3-chloro-5-({1-[(4-methyl-5-oxo-4,5-dihydro-1H-1,2,4-triazol-3-yl)methyl]-2-oxo-4-(trifluoromethyl)-1,2-dihydropyridin-3-yl}oxy)benzonitrile 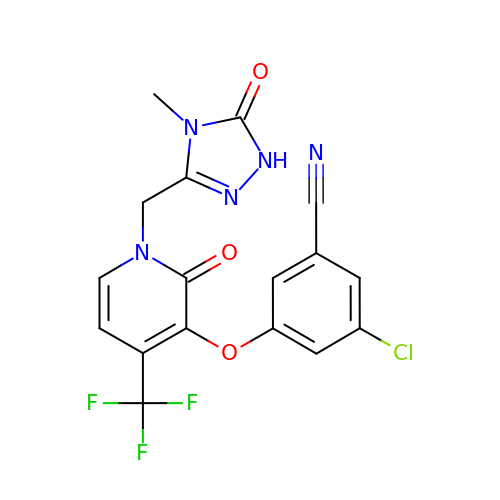| C17 H11 Cl F3 N5 O3 | ZIAOVIPSKUPPQW-UHFFFAOYSA-N> MPRLTTITLYEHDEKRYRDIAGDKKAIQDALIKLNKQFKKDFKKLDRSEDNSDTEDTIDESKGVVEVYANKIKARHYVGFAAVDNVFLQILPKVFKPKKEQTQETQEDTWEPILAFIRMLDMAYGLKIKDHDLAYLQGRNLRPNLYEVFIYLFAKSLWSEVQRGYHREYVEVHREEKFLRGKLLMSRQIRKLPHQLNTFSVEVHELIED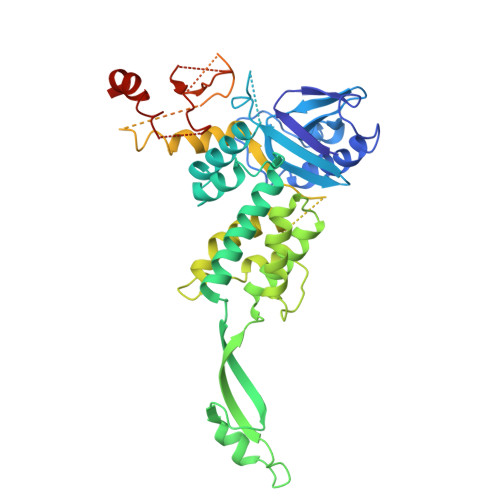NLLNRIFYASVREALRRTTWGLNRKLLGELMLAFDGITPIHLRTEHFERVHFTRLNERFRRPFELAKLLFMPASGKGRSREVSGFFVDMNKLFERFIERVLVRNLPPEYKLFYQESYPFLKNQNGSSQKPDYVVRKGNTPVVVLDAKYRELKERIPSSDMLRQLYVYSRIWGYKTSHENDSKPPAVIVIPSSSTYNQGLPDKPLEFEFFDERKLFIVAYNMDYVKTGAIFKADKNFRRSLNNIIGKLNT> DNLYYWD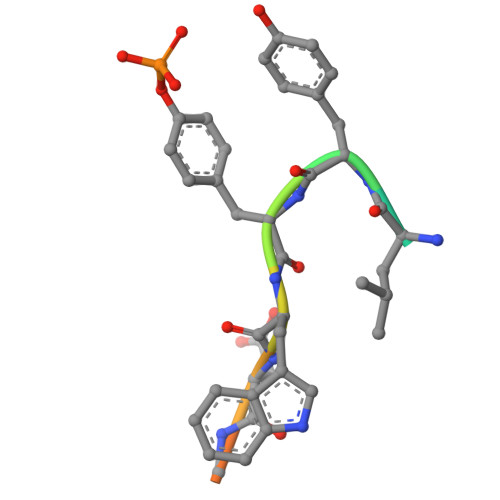QDPP>[2x]DALKVNRAPVGVEPQEVHKWLQSFNWDFKENRTKYPTKYHMANETKEQFKVIAKEYARMEAAKDERQFGTLLDGLTRLGAGNKVHPRWGETMKVISN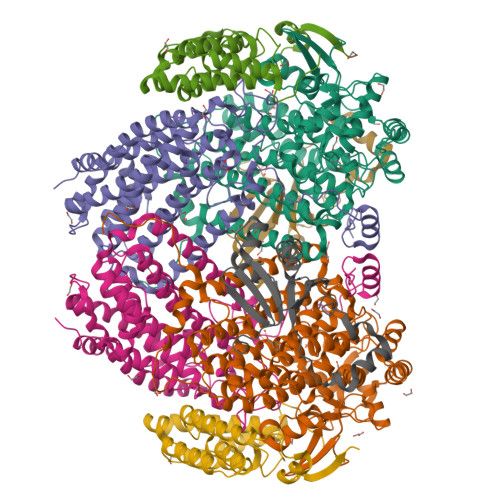FLEVGEYNAIAASAMLWDSATAAEQKNGYLAQVLDEIRHTHQCAFINHYYSKHYHDPAGHNDARRTRAIGPLWKGMKRVFADGFISGDAVECSVNLQLVGEACFTNPLIVAVTEWASANGDEITPTVFLSVETDELRHMANGYQTVVSIANDPASAKFLNTDLNNAFWTQQKYFTPVLGYLFEYGSKFKVEPWVKTWNRWVYEDWGGIWIGRLGKYGVESPASLRDAKRDAYWAHHDLALAAYAMWPLGFARLALPDEEDQAWFEANYPGWADHYGKIFNEWKKLGYEDPKSGFIPYQWLLANGHDVYIDRVSQVPFIPSLAKGTGSLRVHEFNGKKHSLTDDWGERQWLIEPERYECHNVFEQYEGRELSEVIAEGHGVRSDGKTLIAQPHTRGDNLWTLEDIKRAGCVFPDPLAKF;>PQSSQVTKRGLTDPERAAIIAAAVPDHALDTQRKYHYFIQPRWKRLSEYEQLSCYAQPNPDWIAGGLDWGDWTQKFHGGRPSWGNESTELRTTDWYRHRDPARRWHHPYVKDKSEEARYTQRFLAAYSSEGSIRTIDPYWRDEILNKYFGALLYSEYGLFNAHSSVGRDCLSDTIRQTAVFAALDKVDNAQMIQMERLFIAKLVPGFDASTDVPKKIWTTDPIYSGARATVQEIWQGVQDWNEILWAGHAVYDATFGQFARREFFQRLATVYGDTLTPFFTAQSQTYFQTTRGAIDDLFVYCLANDSEFGAHNRTFLNAWTEHYLASSVAALKDFVGLYAKVEKVAGATDRAGVSEALQRVFGDWKIDYADKIGFRVDVDQKVDAVLAGYKN[2x];>[2x]AKREPIHDNSIRTEWEAKIAKLTSVDQATKFIQDFRLAYTSPFRKSYDIDVDYQYIERKIEEKLSVLKTEKLPVADLITKATTGEDAAAVEATWIAKIKAAKSKYEAERIHIEFRQLYKPPVLPVNVFLRTDAALGTVLMEIRNTDYYGTPLEGLRKERGVKVLHLQA;>SSAANAYNAGIMQKTGKAFADEFFAEENQVVHESNAVVLVLMKSDEIDAIIEDIVLKGGKAKNPSIVVEDKAGFWWIKADGAIEIDAAEAGELLGKPFSVYDLLINVSSTVGRAYTLGTKFTITSELMGLDR[2x]ELKS proteins play a key role in organizing intracellular vesicle trafficking and targeting in both neurons and non-neuronal cells. Rab6 is an evolutionarily conserved Rab-GTPase that associates with vesicles and regulates vesicle trafficking to and from the Golgi apparatus. As Rab6 effectors, the scaffold proteins ELKS (also known as Rab6IP2, CAST, or ERC) in vertebrates are encoded by two genes, Erc1 and Erc2, expressing ELKS1 and ELKS2, respectively. The ELKS proteins consist of an N-terminal intrinsic disorder region (IDR), a middle long coiled-coil region and a C-terminal Postsynaptic density-95/Discs large/Zona occludens-1 (PDZ)-binding motif (PBM).

Using high-quality samples of ELKS1_RBD and Rab6BQ72L, we crystallized the ELKS1_RBD/Rab6BQ72L complex and determined the complex structure at 2.04 Å resolution. In the crystal, each asymmetric unit contains two ELKS1_RBD molecules and two Rab6BQ72L molecules, which form two essentially identical complexes with a binding ratio of 1:1 between ELKS1_RBD and Rab6BQ72L. In the complex structure, Rab6BQ72L adopts the typical active GTPase conformation with a bound GTP molecule and ELKS1_RBD consists of two α-helices (αN and αC) to interact with the switch Ⅰ, switch Ⅱ, and interswitch regions of Rab6BQ72L. The two helices in ELKS1_RBD fold as a helical hairpin through interhelical hydrophobic interactions, which resembles the coiled-coil conformation and explains the monomer instead of dimer formation of this predicted coiled-coil region. The binding of ELKS1_RBD to Rab6BQ72L involves both polar and hydrophobic interactions. Specifically, four pairs of charged residues (E857ELKS1-R84Rab6B, E869ELKS1-K13Rab6B, D871ELKS1-R63Rab6B, and K905ELKS1-D49Rab6B) form salt bridges to stabilize the interaction between ELKS1 and Rab6B. Among these charged residues, D871ELKS1 and K13Rab6B are further involved in the hydrogen bond network connected by S868ELKS1 and Q65Rab6B, which further strengthens the binding of ELKS1_RBD to Rab6BQ72L. In addition to the polar interactions, several hydrophobic residues in ELKS1_RBD, including L864, I867, T908, and M912, pack with the hydrophobic pocket formed by the switch II and interswitch regions of Rab6B. Compared to the other Rab6 effectors, ELKS1 occupies a larger surface on Rab6, encompassing not only the switch regions but also the interswitch region. The extended part of ELKS1_RBD interacts with a region outside the canonical effector binding site, specifically, the residues L11 and K13 in the β1-strand of Rab6BQ72L, which are strictly conserved in Rab6 family members but not in other Rab members.

>[2x]GPGSGNPLRKFKLVFLGEQSVGKTSLITRFMYDSFDNTYQATIGIDFLSKTMYLEDRTVRLQLWDTAGLERFRSLIPSYIRDSTVAVVVYDITNLNSFQQTSKWIDDVRTERGSDVIIMLVGNKTDLADKRQITIEEGEQRAKELSVMFIETSAKTGYNVKQLFRRVASALPG;>GPGSRKHLEEVLEMKQEALLAAISEKDANIALLELSSSKKKTQEEVAALKREKDRLVQQLKQQTQNRMKLMADNYEDD[2x]>[2x]GPLGSPVVVRGWLHKQDSSGMRLWKRRWFVLADYCLFYYKDSREEAVLGSIPLPSYVISPVAPEDRISRK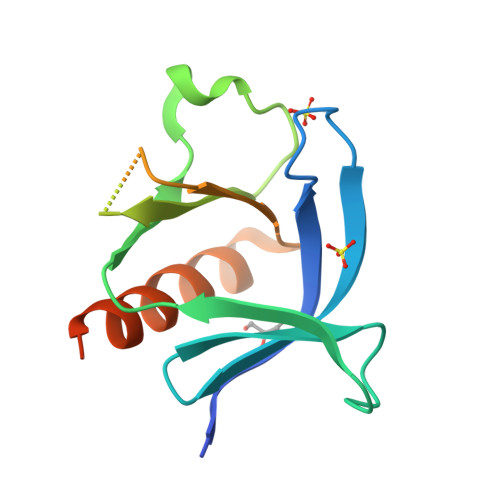YSFKAVHTGMRALIYNSSTAGSQAEQSGMRTYYFSADTQEDMNAWVRAMNQAAQVLSRSSLKRDMEKVER Transient receptor potential (TRP) channels are polymodal molecular sensors involved in numerous physiological processes and implicated in a variety of human diseases. Here, we present structures of the full-length thirteen-lined ground squirrel TRPV1 solved by cryo-EM. Our structures resolve the extracellular cap domain formed by the S5-P-loops and the C-terminus that wraps around the three-stranded β-sheet connecting elements of the TRPV1 intracellular skirt. The cap domain forms a dome above the pore’s extracellular entrance, with four portals leading to the ion conductance pathway.

The apo-state structure of the full-length sqTRPV1 shows at least nine well-resolved densities of annular lipids per channel subunit. The majority of densities have a clear head-and-two-tails appearance and were modelled with phosphatidylcholine. In the apo state, the same residues contribute to the binding of PI, which resides deeper in the vanilloid site towards the linker domain and pushes away the side chain of tyrosine Y513. Strong density in the middle of the cap, which we interpreted as a chloride ion coordinated by arginines R624, represents a likely barrier for cation conductance along the central axis of the channel. The cryo-EM density for the cap is relatively weak and is completely missing for residues 608–617. This can be explained by the dynamic nature of the S5-P-loops and by possible spontaneous crosslinking of cysteines C623, which in the fourfold symmetrical model of sqTRPV1 come close together at the centre of the cap with 5.5 Å distances between their Cα atoms. The C-terminus of sqTRPV1 represents an extended polypeptide that wraps around the three-stranded β-sheet, which connects the ankyrin repeat domains of the neighbouring subunits to form the typical for TRPV channels intracellular skirt. As a result, the intracellular skirt of full-length sqTRPV1 is less dynamic than that of truncated rTRPV1. Indeed, the entire skirt is well-resolved in the cryo-EM density of full-length sqTRPV1, while density for two peripheral of the six ankyrin repeats, as well as the C-terminal hook domain preceding the third strand of the three-stranded β-sheet in truncated rTRPV1 was missing. Other than these differences, apo-state structures of sqTRPV1 and rTRPV1 are quite similar, suggesting that whenever the complete termini are present in rTRPV1, they are likely to interact with the rest of the protein in the same way as in sqTRPV1.

>MKKWANLDSGESEDPPHEDSCPDPPDGDPNSKQSPAKPHIFSTTKSRTRLFGKGDSEEASPMDCSYEEGELASCPTITVSSVVIIQRPGDALTCARQLSQDSVSAGAEKPLKLYDRRSIFDAVAQNNCQELESLLPFLQKSRKRLTDSEFKDPETGKTCLLKAMLNLHNGQNDTISLLLDIARQTDSLKEFVNASYTDSYYKGQTALHIAIERRNMALVTLLVENGADVQAAANGDFFKKTKGRPGFYFGELPLSLAACTNQLAIVKFLLQNSWQPADISARDSVGNTVLHALVEVADNTADNTKFVTSMYNEILILGAKLHPTLKLEELINKKGLTPLALAASSGKIGVLAYILQREIQEPECRHLSRKFTEWAYGPVHSSLYDLSCIDTCEKNSVLEVIAYSSSETPNRHDMLLVEPLNRLLQDKWDRFVKRIFYFNFFVYCLYMIVFTTAAYYRPVDGLPPYKLKNTVGDYFRVTGEILSVSGGVYFFLRGIQYFLQRRPSMKTLFVDSYSEMLFFVQSLFMLGSVVLYFSHRKEYVASMVFSLAMGWTNMLYYTRGFQQMGIYAVMIEKMILRDLCRFMFVYLVFLFGFSTAVVTLIEDGKNYSEPAEYTSHRWRAPGCRPPDSYNSLYSTCLELFKFTIGMGDLEFTENYDFKAVFIILLLAYVILTYILLLNMLIALMGETVNKIAQESKNIWKLQRAITILDTEKSFLKCMRKAFRSGKLLQVGYTPDGKDDYRWCFRVDEVNWTTWNTNVGIINEDPGNCEGVKRTLSFSLRSGRVSGRNWRNFALVPLLRDASTRDRHHAQPEEVHLKHFAGSLKPEDAEVFKDSMAPGEKLPVR[4x]methyl 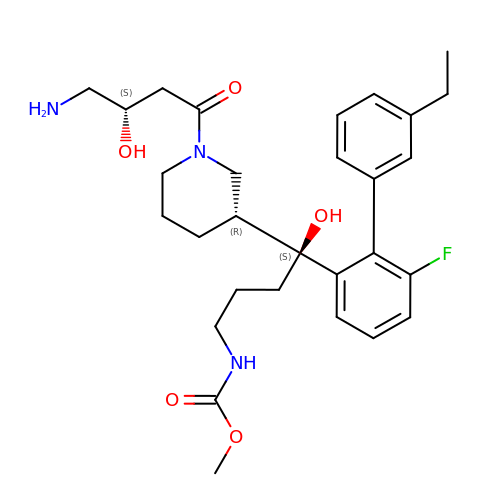[(4S)-4-{(3R)-1-[(3S)-4-amino-3-hydroxybutanoyl]piperidin-3-yl}-4-(3'-ethyl-6-fluoro[1,1'-biphenyl]-2-yl)-4-hydroxybutyl]carbamate | C29 H40 F N3 O5 | IIIBTAZKWKWKNG-AFKLWXAFSA-N4-METHYL-2H-CHROMEN-2-ONE 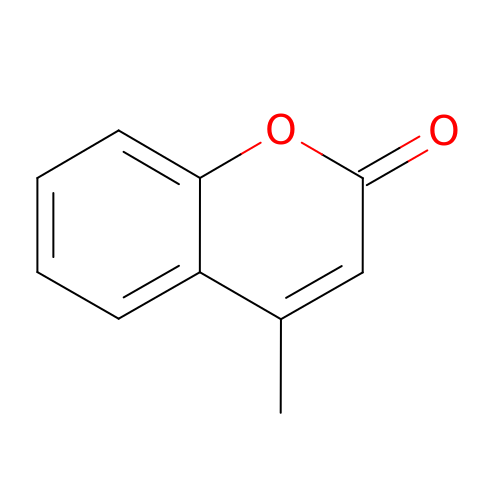| C10 H8 O2 | PSGQCCSGKGJLRL-UHFFFAOYSA-N>[6x]HMSTQPKTLTVGLFPYLPSWNENGNEVKL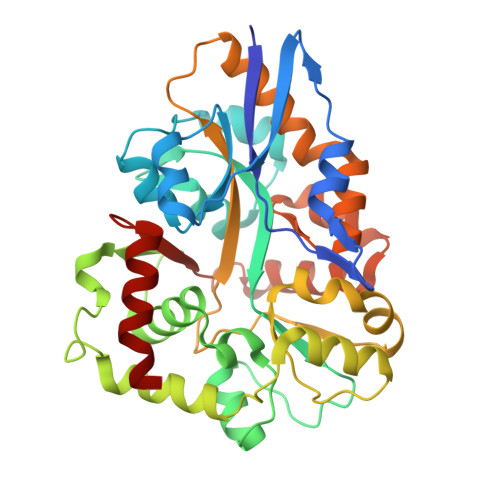INLIKDVLPTQVSGYNIEYTEFDCYSDASLQSLPDVFSTDSIFLPYLVSLGGVKSLDESLVRGVTGDLHSFVSSSASVNGSVYGFPQYLCSNFLLSSPNATQQASSLLELAQKVGYEQIVYPDVASSSSFTVFGLYQQLLQSSSSAAVDIKASDLPQSGDQVNKDITQKYRTILDSTVVASQREYINSVKQGKPISNYYVGYSESMCEIKDIIRDQQYNVQLIGTSDKPYVYTDVLALNSNLCDEKQKVAVEVIKNLLTNTLVLDLLGLGLTLPANKNGIAHLAKSSNFYAQLSQQFDAKESEVRVLRCVDFANKEVKNCAGVLRPFL> 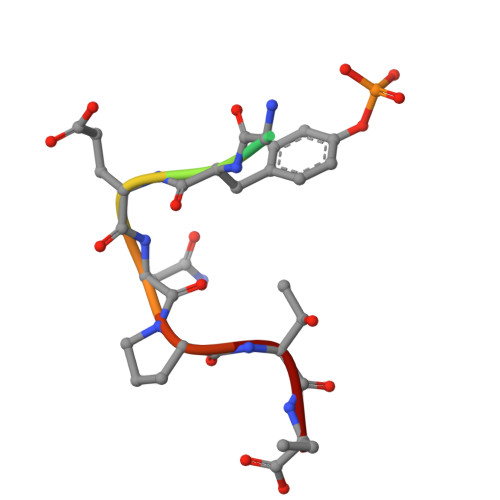QNGYENPTY>EKLGKLQYSLDYDFQNNQLLVGIIQAAELPALDMGGTSDPYVKVFLLPDKKKKFETKVHRKTLNPVFNEQFTFKVPYSELGGKTLVMAVYDFDRFSKHDIIGE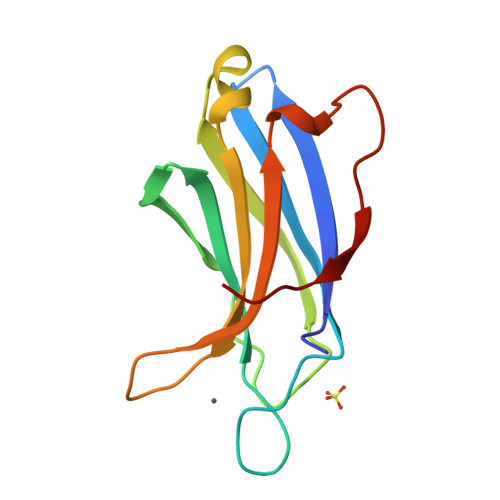FKVPMNTVDFGHVTEEWRDLQSA[2x]2-[4-(1,3-benzothiazol-5-ylamino)-6-~{tert}-butylsulfonyl-quinazolin-7-yl]oxyethyl dihydrogen phosphate | C21 H23 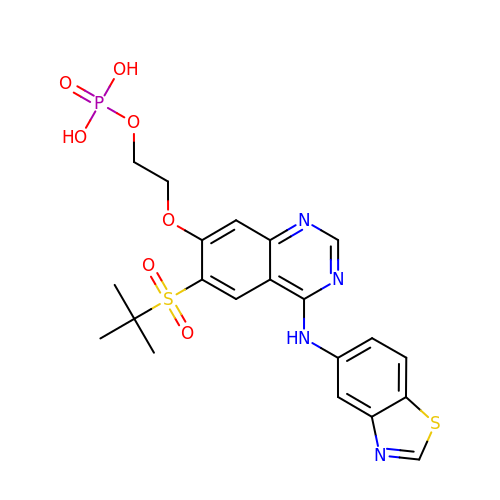N4 O7 P S2 | MJLYDVMFNHZMLV-UHFFFAOYSA-N>[8x]MRRANDPQRREKIIQATLEAVKLYGIHA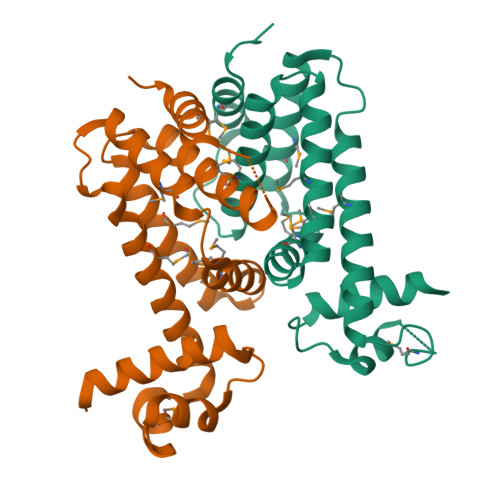VTHRKIATLAGVPLGSMTYYFSGIDELLLEAFSSFTEIMSRQYQAFFSDVSDAPGACQAITDMIYSSQVATPDNMELMYQLYALASRKPLLKTVMQNWMQRSQQTLEQWFEPGTARALDAFIEGMTLHFVTDRKPLSREEILRMVERVAGAAALEHHHHHH> 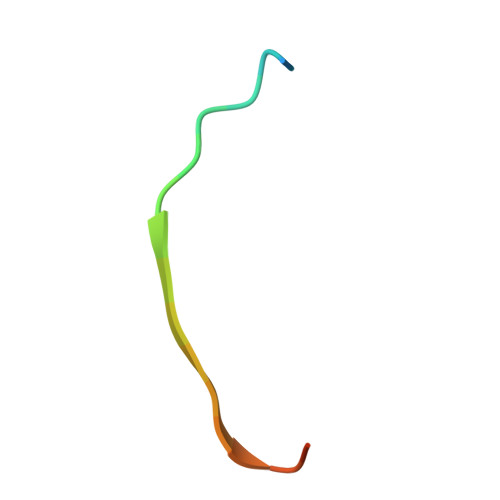NEQSGISQTVIVGPWGAQVST>MRCIGISNRDFVEGVSGGSWVDIVLEHGSCVTTMAKNKPTLDFELIETEAKQPATLRKYCIEAKLTNTTTDSRCPTQGEPSLNEEQDKRFVCKHSMVDRGWGNGCGLFGKGGIVTCAMFTCKKNMKGKVVQPENLEYTIVITPHSGEEHAVGN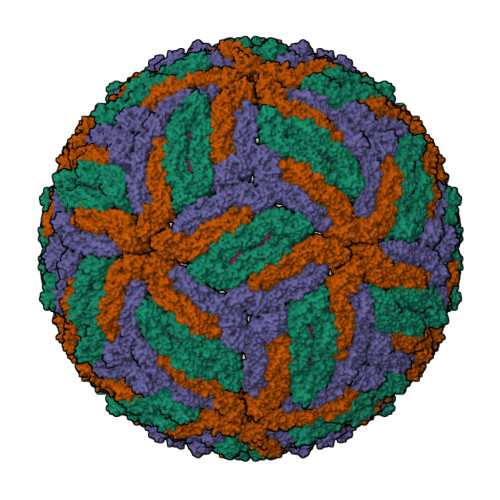DTGKHGKEIKITPQSSITEAELTGYGTVTMECSPRTGLDFNEMVLLQMENKAWLVHRQWFLDLPLPWLPGADTQGSNWIQKETLVTFKNPHAKKQDVVVLGSQEGAMHTALTGATEIQMSSGNLLFTGHLKCRLRMDKLQLKGMSYSMCTGKFKVVKEIAETQHGTIVIRVQYEGDGSPCKIPFEIMDLEKRHVLGRLITVNPIVTEKDSPVNIEAEPPFGDSYIIIGVEPGQLKLNWFKKGSSIGQMIETTMRGAKRMAILGDTAWDFGSLGGVFTSIGKALHQVFGAIYGAAFSGVSWIMKILIGVIITWIGMNSRSTSLSVSLVLVGVVTLYLGVMVQA[3x];>[3x]SVALVPHVGMGLETRTETWMSSEGAWKHAQRIETWILRHPGFTIMAAILAYTIGTTHFQRALIFILLTAVAP> 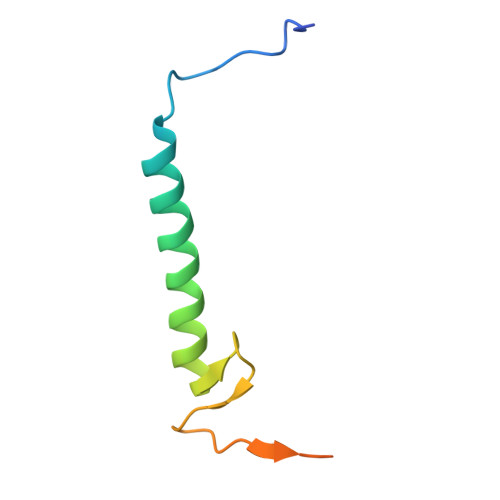GEFKPSACRNLFGPVDHEELTRDLEKHCRDMEEASQRKWNFDFQNHKPLEGKYEWQEVEKGSLPEFYYRPPR>MGSSHHHHHHSSGENLY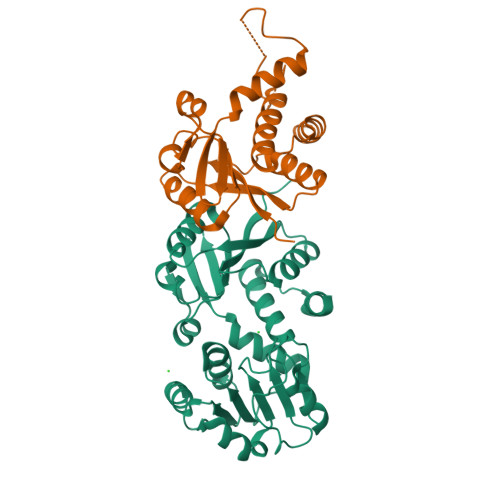FQGHMEKVYGLIGFPVEHSLSPLMHNDAFARLGIPARYHLFSVEPGQVGAAIAGVRALGIAGVNVTIPHKLAVIPFLDEVDEHARRIGAVNTIINNDGRLVGYNTDGLGYVQALEEEMNITLDGKRILVIGAGGGARGIYFSLLSTAAERIDMANRTVEKAERLVREGDERRSAYFSLAEAETRLAEYDIIINTTSVGMHPRVEVQPLSLERLRPGVIVSDIIYNPLETKWLKEAKARGARVQNGVGMLVYQGALAFEKWTGQWPDVNRMKQLVIEALRR[2x]> GHMAKKTYDLLFKLLLIGDSGVGKTCVLFRFSDD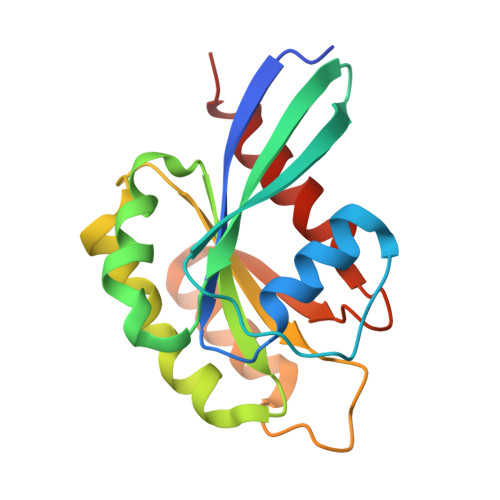AFNTTFISTIGIDFKIKTVELQGKKIKLQIWDTAGQERFHTITTSYYRGAMGIMLVYDITNGKSFENISKWLRNIDEHANEDVERMLLGNKCDMDDKRVVPKGKGEQIAREHGIRFFETSAKANINIEKAFLTLAEDILRKTP> AGMAHAASYLSVGYFNGGGDVTAGPGGDINKLDVTQITHLNYSFGLIYNDEKQETNPALKDPSRLHQIYLSPKVMADLQLLPVLRKQNPELKVLLSVGGWGARGFSGAAATAESRAVFIRSVQQVIKQYHLDGIDLDWEYPVNGAWGLVESQPADRANFTLLLAELHKALDKGKLLTIAVGANVKSPQEWVDVKGIAPYLDYINLMTYDMAYGTQYFNSNLYDSKQWPTVAAADRYSANFVVDNYLAAGLKPAQLNLGIGFYGRVPKRATEPGIDWDKADAAKNPVTQPYFTARETAVFKAMGLDLTKDSYFKYNDIVSKLLNDPQRRFTAHWDSDAQVPYLTMKSAEGKPLFAISYENPRSVALKADYIKSKGLGGAMFWEYGADDNNRLAHQLAESLGINGGKQ

A single-domain GH18 chitinase-D from Serratia proteamaculans (SpChiD) possesses multiple functions, including chitobiase activity to release GlcNAc from CHOS and colloidal chitin, and a hyper-TG activity with CHOS (DP3–6) substrates, generating long-chain CHOS14. Certain chitinases display transglycosylation (TG) activity as well as hydrolysis, forming new glycosidic bonds between donor and acceptor saccharides that can be used for the production of longer-chain and/or well-defined mixtures of CHOS with new or improved biological activities. Catalysis by glycoside hydrolase family 18 (GH18) chitinases proceeds via a substrate-assisted mechanism, which involves an oxazolinium ion intermediate and has a strong preference for a GlcNAc in the –1 subsite. SpChiD displayed an exceptionally high TG activity, in addition to its other inherent functions, and this can be exploited to increase the yield of long-chain CHOS for biological applications.

The SpChiD substrate-binding cleft contains four tryptophan residues (Trp114, Trp160, Trp290 and Trp395) with Trp160 and Trp290 flanking the entrance and Trp114 and Trp395 situated in the catalytic groove of the binding pocket. Half of the space in the SpChiD substrate-binding cleft is occupied by a loop (Asn30–Asp42), and the front face is equipped with Val35 and Thr36, which may provide favorable chemical interactions with the incoming substrate. Phylogenetic analysis of 131 bacterial family-18 chitinases revealed that all the SpChiD-like single-domain chitinases from the Enterobacteriaceae clustered in a distinct group. The novel loop and tryptophan residues were highly conserved in 18 of these enzymes, confirming their divergence from other groups. Therefore, Trp residues at the substrate-binding cleft appear to increase the affinity of substrate binding, thus influencing the TG activity of SpChiD. Mutational analysis also confirmed that Trp114, Trp160 and Trp290 are necessary for TG, and that Trp114 and Trp160 are the most important. The proportion of DP1 produced by SpChiD after 72 h was 96.4%, whereas the mutants V35G, V35F, T36G and T36F produced 54.8%, 96%, 51.4% and 59.5%, respectively. These data suggested the importance of residues Tyr28, Val35, Thr36 and the entire loop in chitobiase activity of SpChiD. SpChiD is active against polymeric substrates, which may depend on the flexible nature of the Asn30-Asp42 loop at the binding cleft. The ability of SpChiD to bind DP2 may favor chitobiase activity over TG activity, whereas perturbations in the positioning or binding of DP2 for chitobiase activity may increase the number of available DP2 molecules at the SpChiD substrate-binding cleft and thus increase TG activity. Further, we conclude that the substrate-binding cleft of a chitinase like SpChiD regulates multiple activities, and could therefore play a similar vital role in the 17 other chitinases present in the same phylogenetic cluster.> QTIQSIPQKGFFGHPRGLGVLFFVEF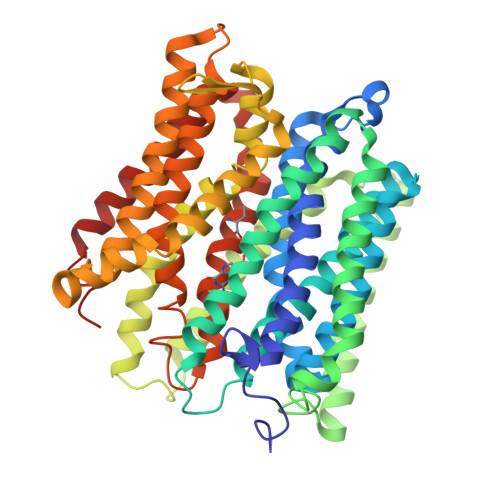WERFSYYGMRAMLIFYMYFAIHQNGLGIDKTTAMSIMSVYGALIYMSSIPGAWIADRITGTRGATLLGAVLIIIGHICLSLPFALFGLFSSMFFIIIGSGLMKPNISNIVGRLYPENDTRIDAGFVIFYMSVNLGALISPIILQHFVDIRNFHGGFLLAAIGMALGLVWYLLFNRKNLGSVGMKPTNPLSKEEKRKYGMIIGIIVAIVIVVLLVTYYTHTLSFDLISNTVLVLGVALPIIYFTTMLRSKDVTDGERSRVKAFIPLFILGMLFWSIQEQGSNVLNIYGLERSDMQLNLFGWTTRFGEALFQSINPLFILLFAPVISMIWLKMGKKQPSLAIKFSIGTLLAGLSYILIGLVGLGYGHTQFSVNWVILSYVICVIGELCLSPTGNSAAVKLAPKAFNAQMMSVWLLTNASAQAINGTLVKLIKPLGQTNYFIFLGTVAIVITLIILVFSPKITKA>CIKGNVDLVFLFDGSMSLQPDEFQKILDFMKDVMKKLSNTSYQFAAVQFSTSYKTEFDFSDYVKRKDPDALLKHVKHMLLLTNTFGAINYVATEVFREELGARPDATKVLIII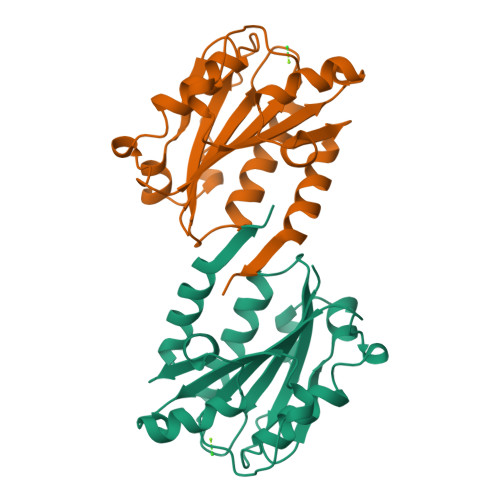TDGEATDSGNIDAAKDIIRYIIGIGKHFQTKESQETLHKFASKPASEFVKILDTFEKLKDLFTELQKKIYVIEG[2x]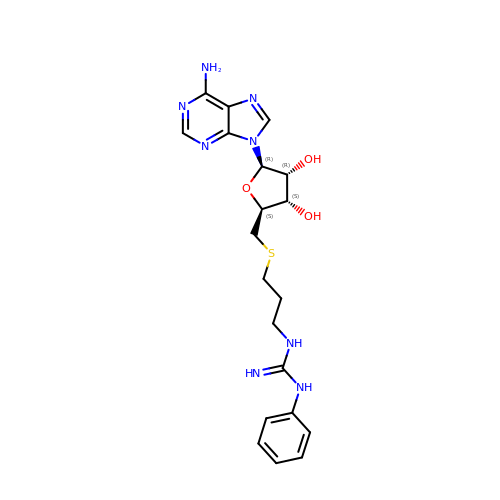5'-S-[3-(N'-phenylcarbamimidamido)propyl]-5'-thioadenosine | C20 H26 N8 O3 S | PAOYFGCZLHEXFB-NVQRDWNXSA-N>MSIAVGMIETRGFP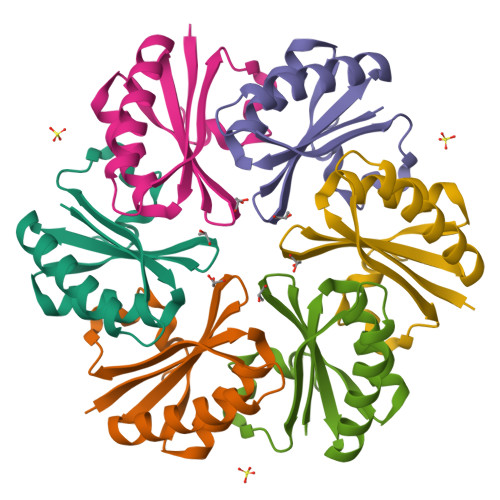AVVEAADSMVKAARVTLVGYEKIGSGRVTVIVRGDVSEVQASVSAGIEAANRVNGGEVLSTHIIARPHENLEYVLPILEHHHHHH[3x]> MNQLFSQGGKGSAGILTNKQAVARHFGVKQSEVVYFSVGVDISGYKVIYDKTTQRAYSLPIG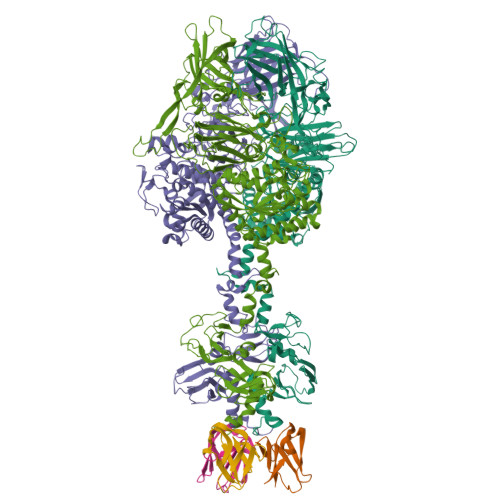IPAGTTAISLSTAAVLVHSQGSVDLGAVAVLRKEYVTIPGDFTSGATIQVKNEILTHSNGAQYRWAGAVPKVVPAGSTPASSGGISASAWIEVTGEELRDELATTGGASQIGTSDGKTVQQWIIANDSANYRARNIQKLAWVDKQVHSRGSIKVLFQGDSMTAGYDTTSTDRVPANNGDWATHASMTYPQRFMAYLPEQSGCSVTGVYRAISGHTAIQSYNEPSWQSNPNCDVVILMLGLNDAGGVAGTTEDIYMEYMEKLIRRFIDWGMGVVVQTCSTGGQGSGGVVANLWAKRMRMMADTYGCAHFNADEVQYYRHNGAVQSDGGHFNSMGYAIHGQMLASMFMAGGLLPTYRPLTNEINTWCGRLDDSIGYCDATGNINLGRSDGAYTRTKVVGGMLANVASIATFSFYLDAEAAHIFVHGSGAGPINVLVDAPSWWNNGAQDYYDFANNQSINFSNSPQAANNAIVDLSTTYSADRKFVGRILGRGWKTLTFFTNLQGTGGDFYLNSLTVQPVPVGMSVQARNWARFDKGHRAVYSKKIPQAYNQATLPTATALVNFQVPMPQSMLPTTPSISGDLGTNFYNCGHSVLKISNSSGDYLEVLLIKTTGGGYVFTGKILKTTYATGNQPTAITATAAHYSMKDLKVAGANGPNMPLETIRDIDMASYVTIGVGAGNGGLVLDINITWPSTPPTSYWNIELEAWDMFGNSEASI;> MIRTTNTCCGNQAGMVEKFIGTAYDVVKTVYDNLGEIQFIYNFLNDYGVLITVDSVTELQELPTTAKYTRVYSSTPTGVRIYTDYLYVEGDRTGVLPSDPTATGSWVVVGSSNSGAATGTGAYIPFVFNNGSAAGGETTIVVPDYTIGVPEIYVEGFRQQVGRGFTFNSVNLTVTLAQPLEQGDEVVLMLSGNPAVPDNPNIDSWTVINWIYNNGAAVGGEQVIVIPYTFQTVPAIFKNGLRYQGGLSTQSYTVDQDNKRILLTEPLSTNDRLVVQLGGELVTLESPDRSLYEIARATNMKDSEVIKSDNTVETLNGKRILYDIVSQVYYWIPSSVPNNVYIQSVVNGQLTYLPGNIVVTLTPIVTLGLSGTTAQRPIGVLTGTQHFDTTLGKPIWFNGTAWVDSTGAVV>SLIGFLSDRQGFEKQYHDIDLSSFGIREGISEIIASTGFEHPNAAPIGIVMKGERPFVRLFKGSHTWENVLKEKCLASNVVYDPILFVRSTFSDLVPSEFEYVDAGEFKFPVLKEAIAWVVFECINLRNTDQSLVADLV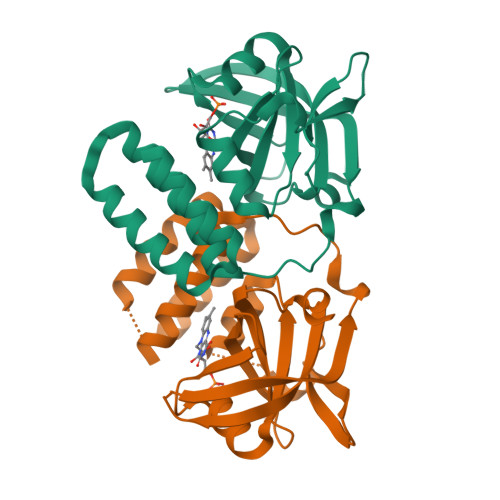PLNAGFNERNIKELPVPNRGFNAVLEATVHATRYQLTGEEKYLELIRHYESLASKCGGDAEKKAMKLIYEALGL[2x]Base excision repair (BER) is the pathway primarily tasked with repairing DNA base damage, with apurinic/apyrimidinic endonuclease (APE1) having both AP-endonuclease and 3′ to 5′ exonuclease (exo) DNA cleavage functions. Importantly, 3′-8-oxoG impairs the ligation step of BER and therefore must be removed by the exo activity of a surrogate enzyme to prevent double stranded breaks and cell death. APE1 has been shown to be the major 3′-exonuclease activity responsible for the repair of 3′-8-oxoG lesions in human cells. APE1 end processing of 8-oxoG, during which the oxidative DNA lesion is removed, results in a ‘clean’ 1-nt gapped substrate suitable for DNA synthesis by Pol β during BER.

To see how the APE1 active site accommodates 3′-8-oxoG, we crystallized APE1 bound with nicked, double stranded DNA substrates containing 8-oxoG at the 3′-end and a phosphate at the 5′-end of the SSB. These substrates represent potentially unligatable, BER intermediates in which the repair polymerase, Pol β, has misinserted an 8-oxodGTP across from either a templating A or C. To obtain crystals of the substrate complexes, we employed a double-mutant catalytically dead variant of APE1 (E96Q/D210N). Specifically, DNA bending at the site of the nick results in an open intra-helical cavity in the DNA, and in both cases the 8-oxoG base is in an anti-conformation and positioned out of the protein active site into the open intra-helical cavity where it does not form any base-pairing interactions with the opposing A or C. This conformation allows the damage-containing 3′ end of the DNA nick and phosphate backbone to shift into the protein active site for cleavage. The 3′-OH of the sugar is also coordinated to N212 (OD1), while the two non-bridging oxygens are coordinated by N212 (ND2), N210 (ND2), Y171 and a water molecule. A second, ordered water molecule is in position to act as the nucleophile. This water is coordinated by the phosphate backbone oxygen (O5′) as well as one of the non-bridging oxygens, positioning the water atom 2.9 Å away from the phosphorus atom. Also observed is a hydrogen bonding network between Q96, D70, N68, N210 and N212 that likely alters the pKa of N210 (D210 in WT APE1), thus facilitating the deprotonation of the water and subsequent nucleophilic attack at the phosphate backbone during cleavage. However, the structure lacks an anticipated bound active site metal ion, which is required for the APE1 exo activity. N174 sits closer to the O8 of O8:A with 2.5 Å between it and the nitrogen (ND2) of the N174A side chain, however in the case of O8:C both the N174 OD1 and ND2 are within hydrogen bonding distance at 2.9 and 3.0 Å, respectively.

>[2x]ALYEDPPDQKTSPSGKPATLKICSWNVDGLRAWIKKKGLDWVKEEAPDILCLQQTKCSENKLPAELQELPGLSHQYWSAPSDKEGYSGVGLLSRQAPLKVSYGIGDEEHDQEGRVIVAEFDSFVLVTAYVPNAGRGLVRLEYRQRWDEAFRKFLKGLASRKPLVLCGNLNVAHEEIDLRNPKGNKKNAGFTPQERQGFGELLQAVPLADSFRHLYPNTPYAYTFWTYMMNARSKNVGWRLDYFLLSHSLLPALCDSKIRSKALGSDHCPITLYLAL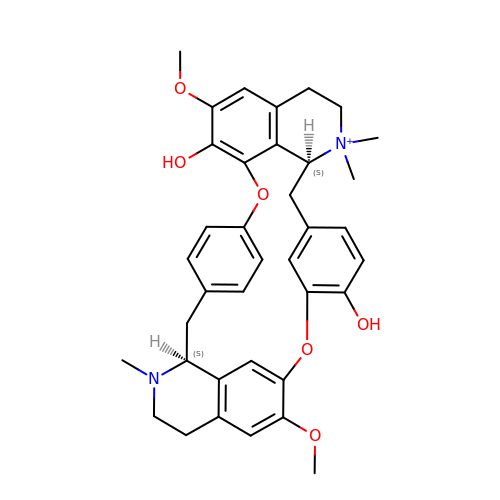(1beta,1'alpha)-7',12'-dihydroxy-6,6'-dimethoxy-2,2',2'-trimethyltubocuraran-2'-ium | C37 H41 N2 O6 | JFJZZMVDLULRGK-VMPREFPWSA-O> GSGMMAEPDPSHPLETQAGKVQEAQDSDSDSEGGAAGGEADMDFLRNLFSQTLSLGSQKERLLDELTLEGVARYMQSERCRRVICLVGAGISTSAGIPDFRSPSTGLYDNLEKYHLPYPEAIFEISYFKKHPEPFFALAKELYPGQFKPTICHYFMRLLKDKGLLLRCYTQNIDTLERIAGLEQEDLVEAHGTFYTSHCVSASCRHEYPLSWMKEKIFSEVTPKCEDCQSLVKPDIVFFGESL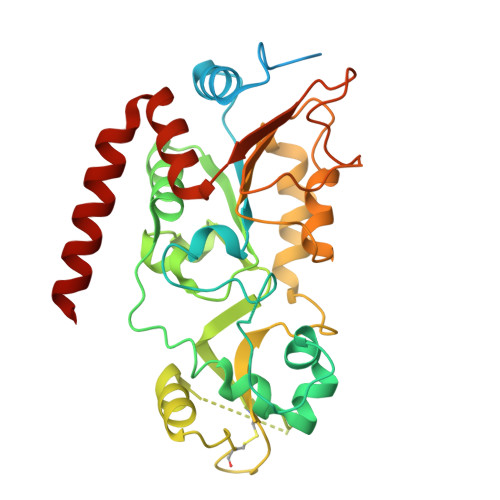PARFFSCMQSDFLKVDLLLVMGTSLQVQPFASLISKAPLSTPRLLINKEKAGQSDPFLGMIMGLGGGMDFDSKKAYRDVAWLGECDQGCLALAELLGWKKELEDLVRREHASIDAQS> GVHKLEPKDHLKPQNLEGISNEQIEPHFEAHYKGYVAKYNEIQEKLADQNFADRSKANQNYSEYRELKVEETFNYMGVVLHELYFGMLTPGGKGEPSEALKKKIEEDIGGLDACTNEL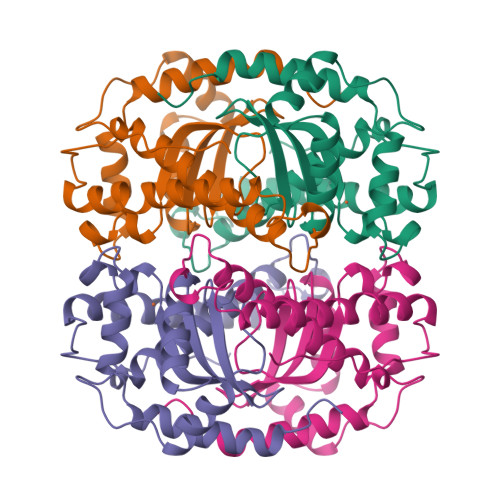KAAAMAFRGWAILGLDIFSGRLVVNGLDAHNVYNLTGLIPLIVIDTYEHAYYVDYKNKRPPYIDAFFKNINWDVVNERFEKAMKAYEALKDFIK4-[[(1~{S})-2-[(~{E})-3-[5-chloranyl-2-(1,2,3,4-tetrazol-1-yl)phenyl]prop-2-enoyl]-3,4-dihydro-1~{H}-isoquinolin-1-yl]carbonylamino]benzoic acid | C27 H21 Cl N6 O4 | 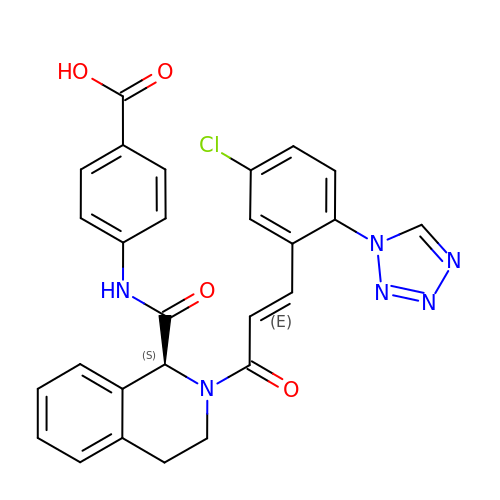XLVCNINDJUKQNE-FRHHVXPKSA-N>[4x]MGHHHHHHMELEGLTALVTGGTSGIGLESARLMAAEGADVVITGRDAQRGEQAAADIGH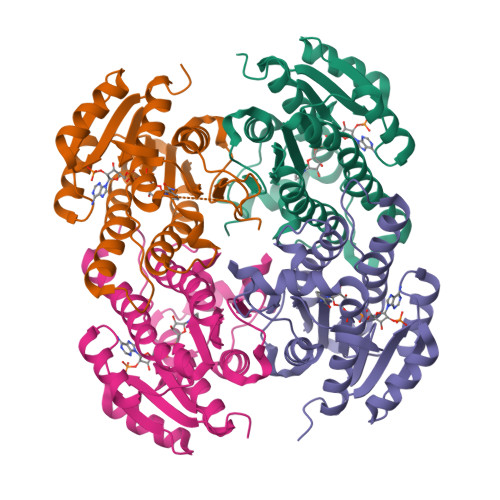GARFVQADLGDLDSVADLAAQAPDVDILVNNAGIYPQASTFDQDVAGFQQLFDTNVRGTYFLVAAAAKGMVARGHGSIVNITTLAAHKGFPGTSVYGATKAALESLTRTWAAEFGANGVRVNSVSPGPTRTPTTLEQLGDFIDDVAAGLPLRRTAAPEEIAQAVLFLASPRASFVTGSTLYVDGGGYAV> TGAGDRHNLKTEWPELVGKSVEEAKKVILQDKPEAQIIVLPVGTIVTMEYRIDRVRL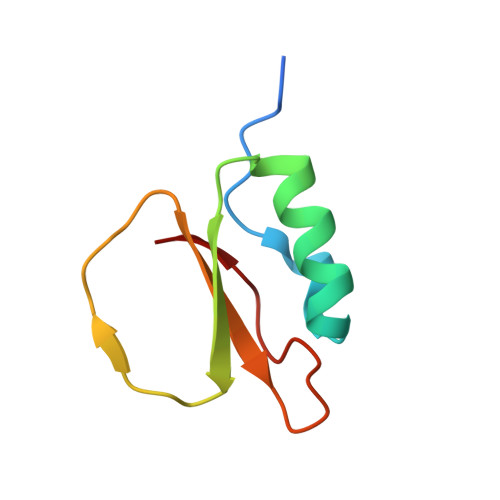FVDKLDNIAEVPRVG> MNNDKRGLNVELSKEISKRVVEHRNRFKRLMFNRYLEFLPLLINYTNRDTVGIDFIQLESALRQNINVVVGEARNKQIMILGYVNNTYFNQAPNFSSNFNFQFQKRLTKEDIYFIVPDYLIPDDCLQIHKLYDNCMSGNFVVMQNKPIQYNSDIEIIEHYTDELAEVALSRFSLIMQAKFSKIFKSEINDESINQLVSEIYNGAPFVKMSPMFNADDDIIDLTSNSVIPALTEMKREYQNKISELSNYLGIN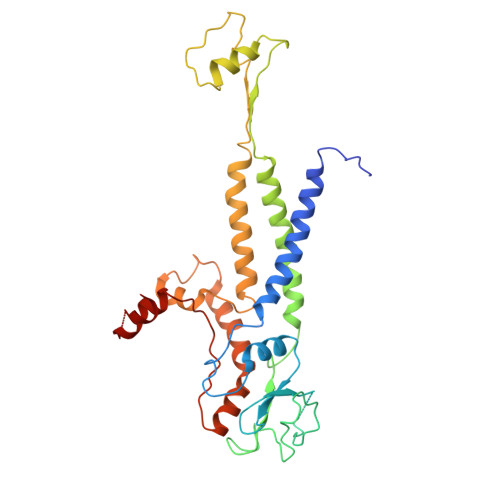SLAVDKESGVSDEEAKSNRGFTTSNSNIYLKGREPITFLSKRYGLDIKPYYDDETTSKISMVDTLFKDESSDING> NTGLLESQLSRHDQMLSVHDIRLADMDLRFQVL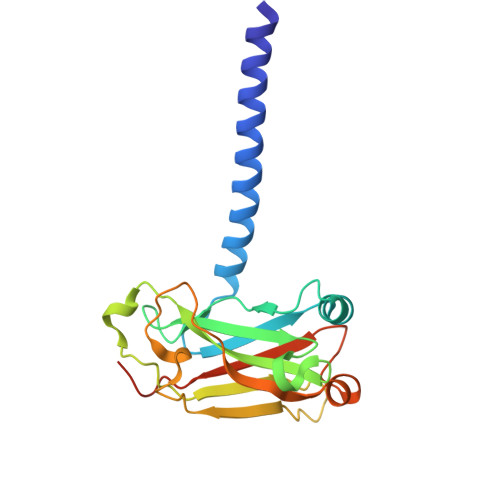ETASYNGVLIWKIRDYKRRKQEAVMGKTLSLYSQPFYTGYFGYKMCARVYLNGDGMGKGTHLSLFFVIMRGEYDALLPWPFKQKVTLMLMDQGSSRRHLGDAFKPDPNSSSFKKPTGEMNIASGCPVFVAQTVLENGTYIKDDTIFIKVIVDTSDLPDPHHHHHH>[2x]MSSKPKYVQDQEMIPGVYWVGIVDWMVRIFHGYHTDEGSSYNSYFIDDECPTVIDSVKYPFAEEWLSRIAACCPLDK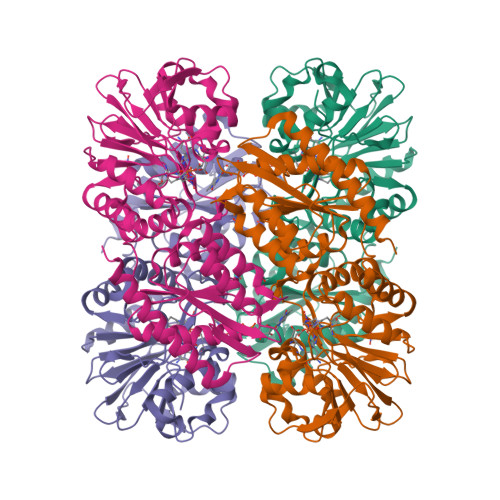IKYVVMNHAEGDHASSLKDHYHKFTNATFVCTKKCQEHLKILYGMEKATWLIVDDKYTLKIGKRTLKFIPVPLLHWPDSTFTYCPEDKILFSNDGFGQHYATSRRWADECDVSHVMHLFKEYTANILGLFSAQMRKALEVASTVEIKYILSAHGVSWRGDAMGLAIAEYDRWSKGQHCQKKVTVVLDSMYGTTHRMALALLDGARSTGCETVLLEMTSSDITKVALHTYDSGAVAFASPTLNNTMMPSVAAALNYVRGLTLIKGKPAFAFGAFGWSNRAVPDIVAELRDGCKADVYDEKGITFKFNYTEELLEQAYNAGVDLGKRAIAYCEKNAPKQ> MAFRKSNVYLSLVNSYIIDSPQPSSINYWWNMGSLLGLCLVIQIVTGIFMAMHYSSNIELAFSSVEHIMRDVHNGYILRYLHANGASFFFMVMFMHMAKGLYYGSYRSPRVTLWNVGVIIFILTIATAFLGYCCVYGQMSHWGATVITNLFSAIPFVGNDIVSWLWGGFSVSNPTIQRFFALHYLVPFIIAAMVIMHLMALHIHGSSNPLGITGNLDRIPMHSYFIFKDLVTVFLFMLILALFVFYSPNTLGHPDNYIPGNPLVTPASIVPEWYLLPFYAILRSIPDKLLGVITMFAAILVLLVLPFTDRSVVRGNT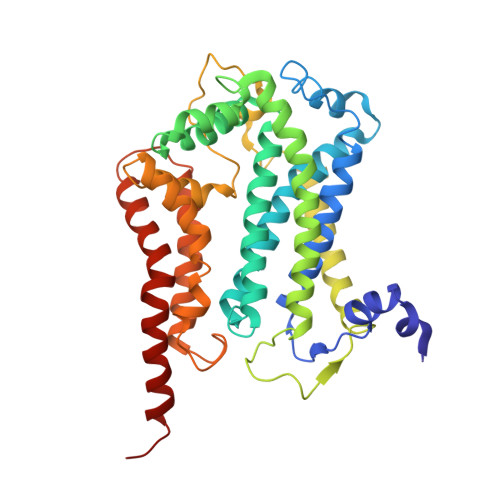FKVLSKFFFFIFVFNFVLLGQIGACHVEVPYVLMGQIATFIYFAYFLIIVPVISTIENVLFYIGRVNK>[8x]MTQPMPGKPAEDAENELDIRGLFRTLWAGKLWIIGMGLAFALIALAYTFFARQEWSSTAITDRPTVNMLGGYYSQQQFLRNLDVRSNMASADQPSV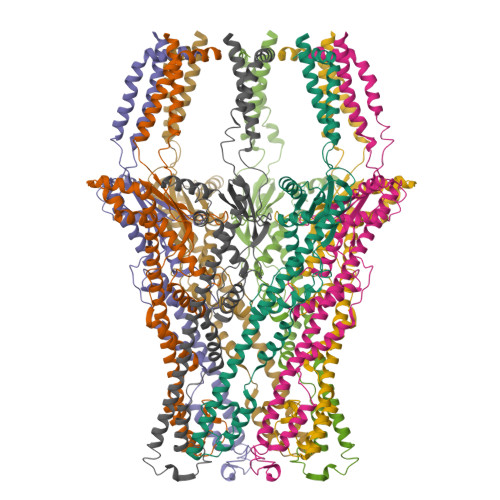MDEAYKEFVMQLASWDTRREFWLQTDYYKQRMVGNSKADAALLDEMINNIQFIPGDFTRAVNDSVKLIAETAPDANNLLRQYVAFASQRAASHLNDELKGAWAARTIQMKAQVKRQEEVAKAIYDRRMNSIEQALKIAEQHNISRSATDVPAEELPDSEMFLLGRPMLQAALENLQAVGPAFDLDYDQNRAMLNTLNVGPTLDPRFQTYRYLRTPEEPVKRDSPRRAFLMIMWGIVGGLIGAGVALTRRCSKEFRVPGSHHHHHHHH Most importantly, the T6SS from the Gram-negative, pathogenic bacterium Pseudomonas aeruginosa was shown to inject at least three different effector molecules (named Tse1, Tse2, and Tse3; Type-6-Secretion-Exported) into the periplasmic space of competing cells. Tse1 was shown to be an amidase that cleaves the γ-D-glutamyl-l-meso-diaminopimelic acid amide bond of crosslinked PG, and Tse3 is a muramidase that cleaves the PG-backbone between the N-acetylmuramic acid and the N-acetylglucosamine moieties. As injection of effector proteins by the T6SS would also cause cell death of siblings, P. aeruginosa co-synthesizes the cognate immunity proteins Tsi1 and Tsi3 (Type-6-Secretion-Immunity) and shuttles them into their periplasmic space to confer resistance. Tse1 adopts the fold of N1pC/P60 papain-like cysteine peptidases, which are widespread among bacteria and of which homologues were identified in eukaryotes, phages, viruses, and archaea.

Interestingly, native Tse1 crystallized under similar conditions but with a different morphology and with a different crystal packing. Thus, phases for the native crystal form were obtained by molecular replacement using the refined model from the selenomethionine-substituted protein structure and refined to 1.7 Å resolution. In both structures, four molecules per asymmetric unit were found which were virtually identical to each other. The core of the protein is formed by a twisted, five-stranded antiparallel β-sheet in a half-barrel configuration. This half-barrel is shielded by surrounding α-helices. Cys30 is found to be in close proximity to a histidine residue (His91), which is the second highly conserved residue within the N1pC/P60 family. Together, Cys30 and His91 form the catalytic diad commonly found in cysteine proteases. Most likely, the deprotonation of the cysteine residue is performed via a water molecule (W1) which is bound between Cys30 and His91 rather than by the histidine residue directly. In our crystal structure of Tse1, a water molecule (W2) was found at this position. However, in Tse1 we observed a cysteine residue at this position, which cannot maintain the correct tautomeric form of His91 with a hydrogen bond, demonstrating that the minimal requirement for N1pC/P60 hydrolases is a Cys-His catalytic diad. However, in the native protein DSB2 was absent.

>MDSLDQCIVNACKNSWDKSYLAGTPNKDNCSGFVQSVAAELGVPMPRGNANAMVDGLEQSWTKLASGAEAAQKAAQGFLVIAGLKGRTYGHVAVVISGPLYRQKYPMCWCGSIAGAVGQSQGLKSVGQVWNRTDRDRLNYYVYSLASCSLPRASAAALEHHHHHH[4x]> GAMGMIDIHSHIVFDVDDGPKSREESKALLAESYRQGVRTIVSTSHRRKGMFETPEEKIAENFLQVREIAKEVASDLVIAYGAEIYYTPDVLDKLEKKRIPTLNDSRYALIEFSMNTPYRDIHSALSKILMLGITPVIAHIERYDALENNEKRVRELIDMGCYTQVNSSHVLKPKLFGERYKFMKKRAQYFLEQDLVHVIASDMHNLDGRPPHMAEAYDLVTQKYGEAKAQELFIDNPRKIVMDQLI

The function of these proteins is crucially dependent on phosphatases, which are homologs of either Cps4B in Gram-positive bacteria or WzbK-30 in Gram-negative bacteria. Since the dephosphorylation of bacterial tyrosine kinases, such as Wzc and CpsCD, is a crucial part in the capsular assembly process in both Gram-negative and Gram-positive bacteria, the phosphatases represent potential targets for drug development efforts. We have thus characterized representatives from each family: Wzb from E. coli K-30 (denoted WzbK-30) and CpsB from S. pneumoniae TIGR4 (denoted Cps4B). Furthermore, we show that both Wzb and Cps4B are capable of completely dephosphorylating full-length Wzc, establishing that Cps4B activity is not confined to its cognate CpsCD complex.

We solved the structure of Cps4B in two crystal forms, P212121 and P43212. Both structures are identical with the exception of loop 169–177, which shows a significant conformational change between the two crystal forms, indicating a degree of flexibility in this part of the structure. The loop is involved in crystal contacts in both structures, but it would protrude into the surrounding solvent if the protein was in solution. Loop βF/α6 shows a significant conformational change between the two crystal forms P212121 and P43212. It is close to the active site and contains several hydrophobic amino acids that could potentially form hydrophobic interactions with the incoming substrate (e.g., Leu172, Phe173 and Tyr177). The loop is not well conserved over its full length, but many Cps4B homologs contain a FG(D/E)K/R motif in this position, where the phenylalanine corresponds to Phe173 of Cps4B. Although this loop could be important in binding the phosphotyrosine, it does not confer any specificity of Cps4B to CpsCD, since our results show that Cps4B readily dephosphorylates Wzc from E. coli K-30.> GSPGIGGGGGGILDSMVEKLGKLQYSLDYDFQNNQLLVGIIQAAELPALDMGGTSDPYVKVFLLPDKKKKFETKVHRKTLNPVFNEQFTFKVPYSELGGKTLVMAVYDFDRFSKHDI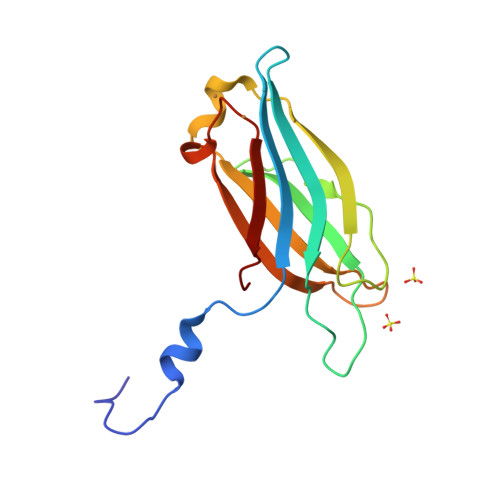IGEFKVPMNTVDFGHVTEEWRDLQSA>SVKLAGNSSLCPVSGWAIYSKDNSVRIGSKGDVFVIREPFISCSPLECRTFFLTQGALLNDKHSNGTIKDRSPYRTLMSCPIGEVPSPYNSRFESVAWSASACHDGINWLTIGISGPDNGAVAVLKYNGIITDTIKSWRNNILRTQESECACVNGSCFTVMTDGPNNGQASYKIFRIEKGKIVKSVEMNAPNYYYEECSCYPDSSEITCVCRDNWHGSNRPWVSFNQNLEYQIGYICSGIFGDNPRPNDKTGSCGPVSSNGANGVKGFSFKYGNGVWIGRTKSISSRNGFEMIWDPNGWTGTDNNFSIKQDI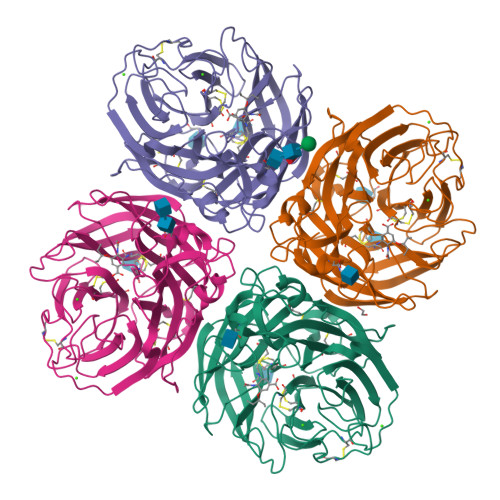VGINEWSGYSGSFVQHPELTGLDCIRPCFWVELIRGRPKENTIWTSGSSISFCGVNSDTVGWSWPDGAELPFTIDK[4x]>[3x]GHMTQAVEAGEKTVEQFVQALNKGDYNKAAEMTSKKAANKSALSEKEILDKYQNIYGAADVKGLQISNLKVDKKDDSTYSFSYKAKMNTSLGELKDLSYKGTLDRNDGQTTINWQPNLVFPEMEGNDKVSLTTQEAARGNIIDRNGEPLATTGKLKQLGVVPSKLGDGGEKTANIKAIASSFDLTEDAINQAISQSWVQPDYFVPLKIIDGATPELPAGATIQEVDGRYYPLGEAAAQLIGYVGDITAEDIDKNPELSSNGKIGRSGLEMAFDKDLRGTTGGKLSITDADGVEKKVLIEHEVQNGKDIKLTIDAKAQKTAFDSLGGKAGSTVATTPKTGDLLALASSPSYDPNKMT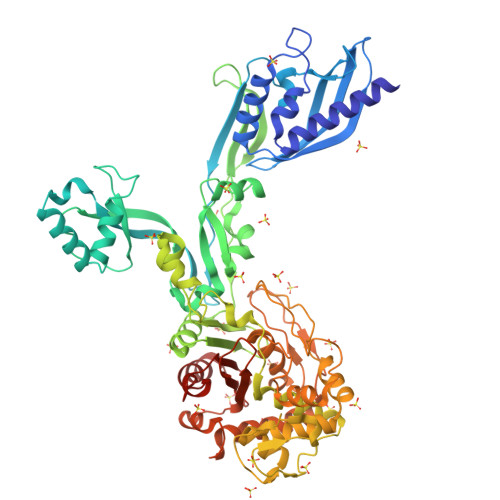NGISQEDYKAYEENPEQPFISRFATGYAPGSTFKMITAAIGLDNGTIDPNEVLTINGLKWQKDSSWGSYQVTRVSDVSQVDLKTALIYSDNIYTAQETLKMGEKKFRTGLDKFIFGEDLDLPISMNPAQISNEDSFNSDILLADTGYGQGELLINPIQQAAMYSVFANNGTLVYPKLIADKETKDKKNVIGETAVQTIVPDLREVVQDVNGTAHSLSALGIPLAAKTGTAEIKEKQDVKGKENSFLFAFNPDNQGYMMVSMLENKEDDDSATKRASELLQYLNQNYQ> GPRLSR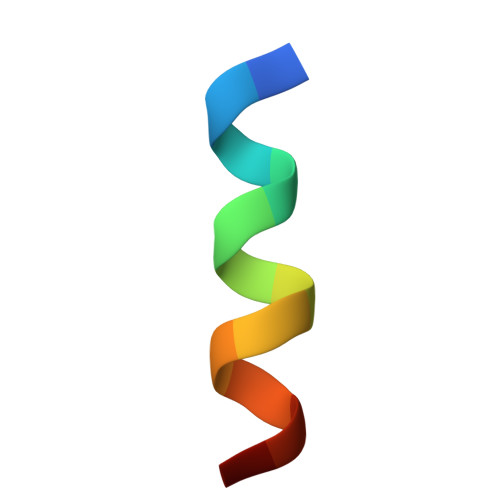LLSSAGC> GFGCNGPWDEDDM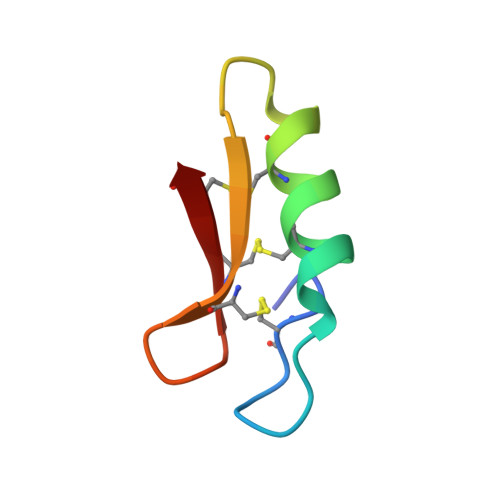QCHNHCKSIKGYKGGYCAKGGFVCKCY> GSDHVISYYHVASDTEKIIREGPTGRLEEYLGSMAKIQKAVEYFQDNSPDSPELNKVKLLFERGKESLESEFRSLMTRHSKVVSPVLLLDLISADDELEVQEDVVLEHLPESVLRDVVRISRWLVEYGRNQDFMNVYYQIRSSQLDRSIKGLKEHFRKSSSSSGVPYSPAI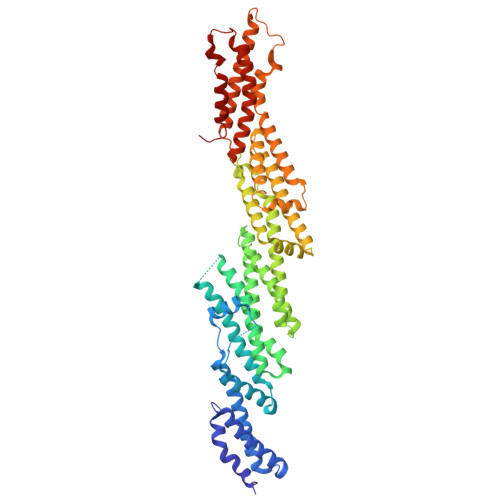PNKRKDTPTKKPIKRPGRDDMLDVETDAYIHCVSAFVKLAQSEYRLLMEIIPEHHQKKTFDSLIQDALDGLMLEGENIVSAARKAIIRHDFSTVLTVFPILRHLKQTKPEFDQVLQGTAASTKNKLPGLITSMETIGAKALEDFADNIKNDPDKEYNMPKDGTVHELTSNAILFLQQLLDFQETAGAMLASQETSSSATSYSSEFSKRLLSTYICKVLGNLQLNLLSKSKVYEDPALSAIFLHNNYNYILKSLEKSELIQLVAVTQKTAERSYREHIEQQIQTYQRSWLKVTDYIAEKNLPVFQPGVKLRDKERQMIKERFKGFNDGLEELCKIQKVWAIPDTEQRDKIRQAQKDIVKETYGAFLHRYGSVPFTKNPEKYIKYRVEQVGDMIDRLFDTSA>MSPSAVQSSKLEEQSSEIDKLKAKMSQSASTAQQKKEHEYEHLTSVKIVPQRPISDRLQPAIATHYSPHLDGLQDYQRLHKESIEDPAKFFGSKATQFLNWSKPFDKVFIPDSKTGRPSFQNNAWFLNGQLNACYNCVDRHALKTPNKKAIIFEGDEPGQGYSITYKELLEEVCQVAQVLTYSMGVRKGDTVAVYMPMVPEAIITLLAISRIGAIHSVVFAGFSSNSLRDRINDGDSKVVITTDESNRGGKVIETKRIVDDALRETPGVRHVLVYRKTNNPSVAFHAPRDLDWATEKKKYKTYYPCTPVDSEDPLFLLYTSGSTGAPKGVQHSTAGYLLGALLTMRYTFDTHQEDVFFTAGDIGWITGHTYVVYGPLLYGCATLVFEGTPAYPNYSRYWDIIDEHKVTQFYVAPTALRLLKRAGDSYIENHSLKSLRCLGSVGEPIAAEVWEWYSEKIGKNEIPIVDTYWQTESGSHLVTPLAGGVTPMKPGSA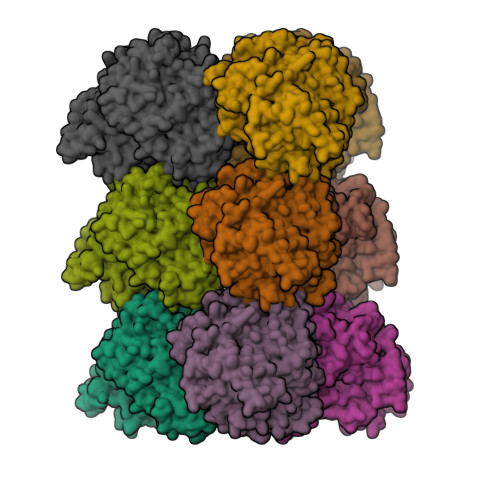SFPFFGIDAVVLDPNTGEELNTSHAEGVLAVKAAWPSFARTIWKNHDRYLDTYLNPYPGYYFTGDGAAKDKDGYIWILGRVDDVVNVSGHRLSTAEIEAAIIEDPIVAECAVVGFNDDLTGQAVAAFVVLKNKSNWSTATDDELQDIKKHLVFTVRKDIGPFAAPKLIILVDDLPKTRSGKIMRRILRKILAGESDQLGDVSTLSNPGIVRHLIDSVKL[9x]(4R,5S)-4-fluoro-1-[(4-fluorophenyl)sulfonyl]-5-methyl-N-({5-(trifluoromethyl)-2-[2-(trifluoromethyl)pyrimidin-5-yl]pyridin-4-yl}methyl)-L-prolinamide 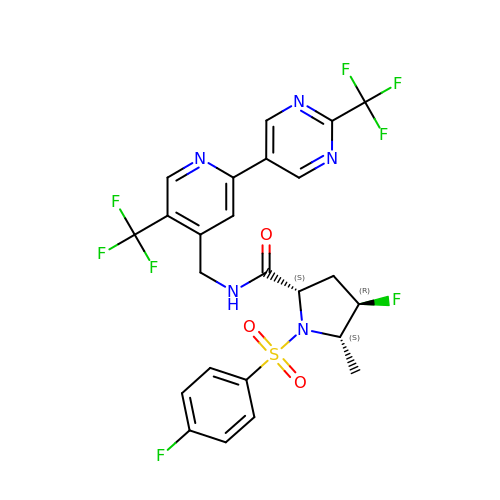| C24 H19 F8 N5 O3 S | RGXNECXVRZKGGH-UOXRKKOCSA-N> VGSLNCIVAVSQNMGIGKNGDFPWPPLRNEFRYFQRMTTTSSVEGKQNLVIMGKKTWFSIPEKNRPLKGRINLVLSRELKEPPQGAHFLSRSLDDALKLTEQPELANKVDMVWIVGGSSVYKEAMNHPGHLKLFVTRIMQDFESDTFFPEIDLEKYKLLPEYPGVLSDVQEEKGIK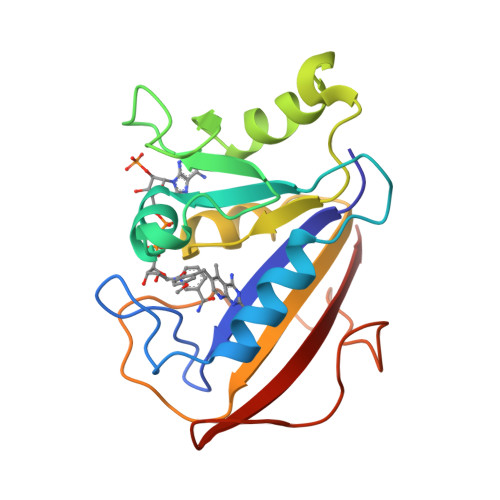YKFEVYEKND> GSMAMKITSSNFATIATSENFAKLSVLPKNHREPIKGLFKSAVEQFSSARDFFKNENYSKELAEKFNKEAVNEAVEKLQKA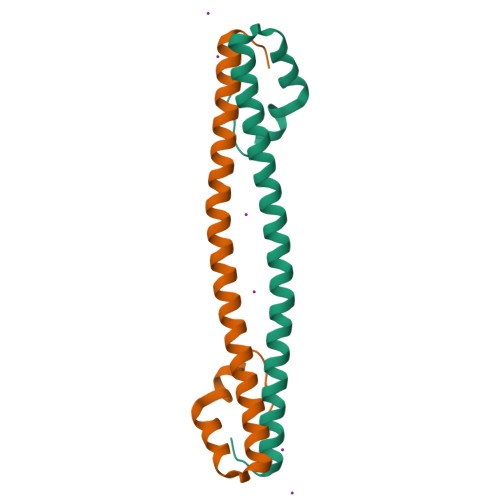IDLAEKQGIQF> LGSRVTMNEFEYLKLLGKGTFGKVILVKEKATGRYYAMKILKKEVIVAKDEVAHTLTENRVLQNSRHPFLTALKYSFQTHDRLCFVMEYANGGELFFHLSRERVFSEDRARFYGAEIVSA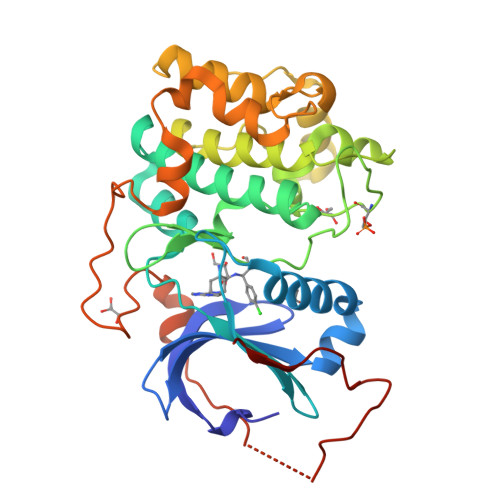LDYLHSEKNVVYRDLKLENLMLDKDGHIKITDFGLCKEGIKDGATMKTFCGTPEYLAPEVLEDNDYGRAVDWWGLGVVMYEMMCGRLPFYNQDHEKLFELILMEEIRFPRTLGPEAKSLLSGLLKKDPKQRLGGGSEDAKEIMQHRFFAGIVWQHVYEKKLSPPFKPQVTSETDTRYFDEEFTAQMITITPPDQDDSMECVDSERRPHFPQFDYSASSTA> MSLKIVFAGTPQFAVPTLRALIDSSHRVLAVYTQPDRPSGRGQKIMESPVKEIARQNEIPIIQPFSLRDEVEQEKLIAMNADVMVVVAYGLILPKKALNAFRLGCVNVHASLLPRWRGAAPIQRAILAGDRETGISIMQMNEGLDTGDVLAKSACVISSEDTAADLHDRLSLIGADLLLESLAKLEKGDIKLEKQDEASATYASKIQKQEALIDWRKSAVEIARQVRAFNPTPIAFTYFEG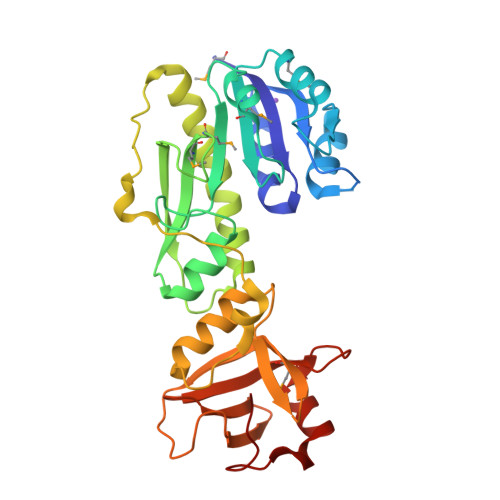QPMRIWRATVVDEKTDFEPGVLVDADKKGISIAAGSGILRLHQLQLPGKRVCSAGDFINAHGDKLIPGKTVFG>PEEVVLDATSPSERLILSPKAKLHVNNGKDVNKGDLIAEEPPIYARRSGVIVDVKNVRKIVVETIDRKYTKTYYIPESAGIEPGLRVGTKVKQGLPLSKNEEYICELDGKIVEIERMKKVVVQTPDGEQDVYYIPLDVFDRDRIKKGKEVKQGEMLAEARKFFAKVSGRVEVVDYSTRKEIRIYKTKRRKLFP[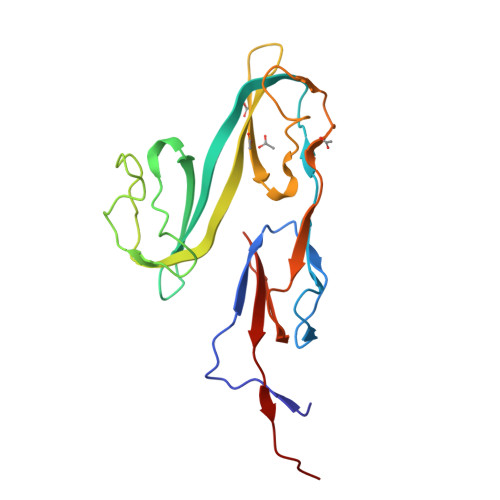2x]> QEDFPPRIVEHPSDLIVSKGEPATLNCKAEGRPTPTIEWYKGGERVETDKDDPRSHRMLLPSGSLFFLRIVHGRKSRPDEGVYVCVARNYLGEAVSHNASLEVAILRDDFRQNPSDVMVAVGEPAVMECQPPRGHPEPTISWKKDGSPLDDKDERITIRGGKLMITYTRKSDAGKYVCVGTNMVGERESEVAELTVLERPSFVKRPSNLAVTVDDSAEFKCEARGDPVPTVRWRKDDGELPKSRYEIRDDHTLKIRKVTAGDMGSYTCVAENMVGKAEASATLTVQEPPHFVVKPRDQVVALGRTVTFQCEATGNPQPAIFWRREGSQNLLFSYQPPQSSSRFSVSQTGDLTITNVQRSDVGYYICQTLNVAGSIITKAYLEVTG

Roundabout (Robo) receptors provide an essential repulsive cue in neuronal development following Slit ligand binding. The Drosophila and vertebrate Robo1-3 are most similar, containing five immunoglobulin (Ig) and three fibronectin (Fn) domains in their extracellular region. Here we present the crystal structure of Robo1 Ig1-4 and Robo1 Ig5, together with a negative stain electron microscopy reconstruction of the Robo1 ectodomain. These results show how the Robo1 ectodomain is arranged as compact dimers, mainly mediated by the central Ig domains, which can further interact in a “back-to-back” fashion to generate a tetrameric assembly.

The Robo1 Ig1-4 domains are arranged in an extended conformation, ∼170 Å in length, with essentially no polypeptide linker between any of the four domains. Two potential N-glycosylation sites at N160 and N175 were identified by sequence analysis. A close inspection of the electron density for these residues reveals clear glycosylation at N160, while N175 is most likely not glycosylated. Nevertheless, four crystallographic contact interfaces are observed. The first results in a dimeric arrangement between 2-fold symmetric molecules along the b axis, and is primarily mediated by the Ig4 domain. This interface, which spans residues 378–394 and 429–436, has the largest buried surface (663 Å2 of each molecule's surface area), and is predominantly hydrophobic in nature. The last interface, which buries 466 Å2 from each molecule, is mediated exclusively by residues 71–72, 86–96, and 122–126 from one Ig1 domain interacting with residues 79–84, 115–120, and 128–131 from the second Ig1. Both interaction surfaces partially overlap with the Slit2 D2 binding surface on Ig1, but Slit2 D2 binding to the first is more extensive compared with the second. Several independent ab initio runs yielded reproducible molecular shapes, and the average models generated are consistent with the Robo1 Ig1-4 structure obtained. The fit directly computed from the atomic model of Robo1 Ig1-4 yields a very good agreement with the experimental SAXS profile and a χ2 = 1.4.> AMDKSAKAPVITIFDHRGCSRAPKE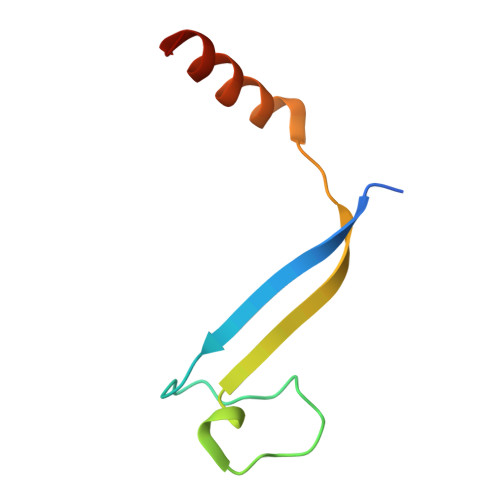YTGSKASGQDDEMMVKAQSVKIAVSDGVAESVLKDSLSVMHK> GGSPINCEKRENLLPFVGLNNLGNTCYLNSILQVLYFCPGFKSGVKHLFNIISRKKEALKSLASYELICSLQSLIISVEQLQASFLLNPEKYTDELATQPRRLLN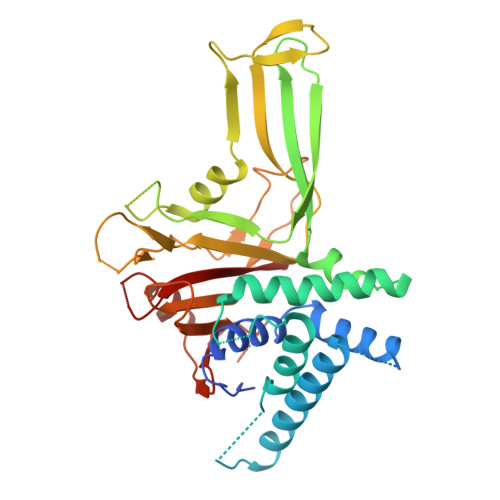TLRELNPMYEGYLQHDAQEVLQCILGNIQETCQLLKKEEVKNVAENEVKPINKGEEQIGFELVEKLFQGQLVLRTRCLECESLTERREDFQDISVPVQEDELSKVEESSEISPEPKTEMKTLRWAISQFASVERIVGEDKYFCENCHHYTEAERSLLFDKMPEVITIHLKCFAASGLEFDCYGGGLSKINTPLLTPLKLSLEEWSTKPTNDSYGLFAVVMHSGITISSGHYTASVKVTDLNSLEQSLKEYEGKWLLFDDSEVKVTEEKDFLNSLSPSTSPTSTPYLLFYKKL> MSIRGTSGSTVARPRLFRTVMTETINGINAEDRYPNSGEVSQLDQFFGDGQRRIAIVAKLTENAEMIVSRAANRIFVGGSPMAYSERQKAKAKSPLANDEFGNEPIVEDRGGFLESLKSIFSTRGGGGRASADFAVPPDFEPINIARYGPERMQKSIRDLDWFLRYTTYAILAGDPSILEANCLGLREILEKSCSISATIVALLEMRKNAARLFKDEADSKLVSSYISVVIRALDADRSDAPADIVRPSSEDRPGLTLPYIYKLSADSLTTFKMTAIYGADGRPKVNLSSDEKERVVRAAYRQVFERDLKAYGQSVSEAESKVKNGEISVREFVRRLGKSELYRREFYQPFINSRVLELAFKHFLGRAPESRAEVQKYFSIISSPIVRGQSSMPSGGLYALIDALIDSEEYTSIFGEDTV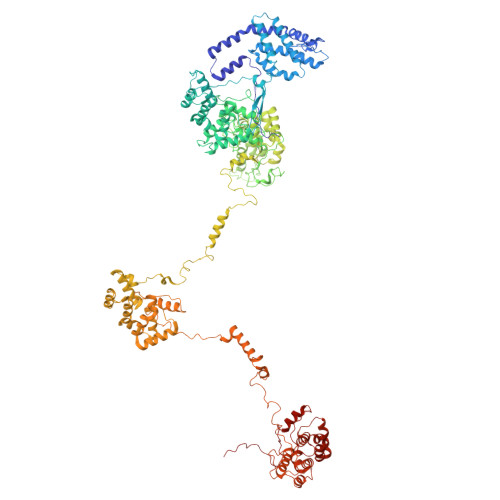PYLRNLGVEAQPSWNWGAAYDLYNYAAPRRKVPQFITLFADYTQPLPNQHPYGAGNDPLEIQFGAIFKNSTINPAERAAPIGKDVKRILIRNGSPTSNERGNPTGMSEGATTLGPKIFKLTQNVGFRSKGMVQNAGVVTVEGSVQALITAAYQQIFGRQLYQGQRLKVAEIKLENGETTVKEFVRALGRSEIFRKLYWEPFYVCKAIEYIHRRLLGRPTYDRVENNRYFDIASKKGFYGVVDAMLNSNEYQEVFGEDVLPYERYLTPAGLSLRKGRFGSSDVLTTPGGITPRGDAARMMDKIQELGTPINERSIPEMYVNQGVPALKRQRKVFKQSQATDRESFDALVTAAYVQVFDKDIASYIRSEFSALESRLRNRETSVKEFVRLLGFSALYRKQFHDRYPNTKVVEFAFKHFLGRAVKNQAELIKYHGLLGRKGIKALIGALVDGEEYGRLYGEDTVPSWQFPTLPAANYPNSVELYNRFTRQDDSLVVPSFKPIRSKMDIASMPLVQAALKEQQATKTALDMSRPMFLELGRSFKGADGQSVEVGVGTLRRQLEHIYRIAPDATRSEKDVAINAIYRQVLDVFAGIPPSYLRLSEAESKLKNNEISVREFVRRLGRSENYRKRFFEPYSSPKVVELLTKHFLGRAPISQQEISTYVQILGTKGLAAAVDAIVESPEYLTIFNEDIVPYRRYPTLPAGNYRASVRVNDEELISQSWSSLSPTYTGYQYVTR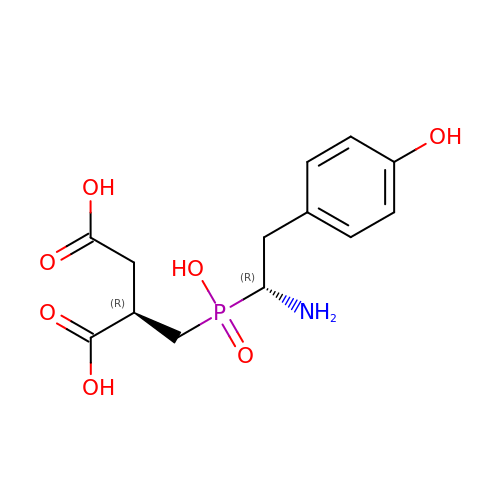(2R)-2-{[(S)-[(1R)-1-amino-2-(4-hydroxyphenyl)ethyl](hydroxy)phosphoryl]methyl}butanedioic acid | C13 H18 N O7 P | UESSIRUCJXFQBC-GXSJLCMTSA-N> FDNPPTNVVSHLNGDWFLFGDSRSDCNHVVNTNPRNYSYMDLNPALCDSGKISSKAGNSIFRSFHFTDFYNYTGEGQQIIFYEGVNFTPYHAFKCTTSGSNDIWMQNKGLFYTQVYKNMAVYRSLTFVNVPYVYNGSAQSTALCKSGSLVLNNPAYIAREANFGDYYYKVEADFYLSGCDEYIVPLCIFNGKFLSNTKYYDD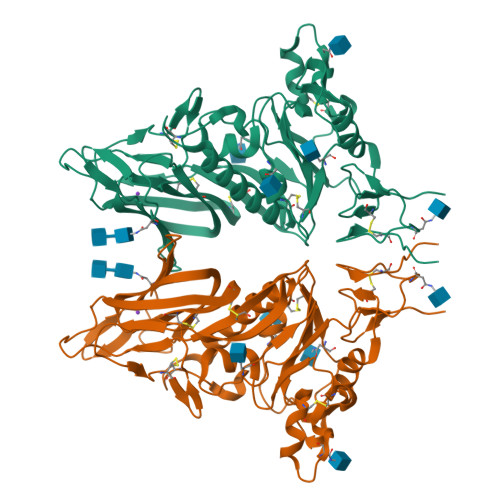SQYYFNKDTGVIYGLNSTETITTGFDFNCHYLVLPSGNYLAISNELLLTVPTKAICLNKRKDFTPVQVVDSRWNNARQSDNMTAVACQPPYCYFRNSTTNYVGVYDINHGDAGFTSILSGLLYDSPCFSQQGVFRYDNVSSVWPLYSYGRCPTAADINTPDVPICVYDSDPLVPR> FMVSLPRMVYPQPKVL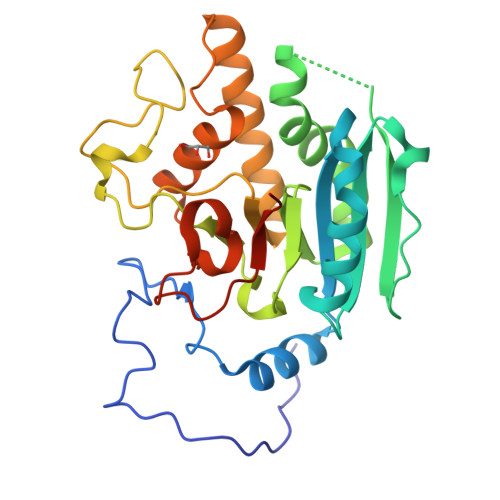TPCRKDVLVVTPWLAPIVWEGTFNIDILNEQFRLQNTTIGLTVFAIKKYVAFLKLFLETAEKHFMVGHRVHYYVFTDQPAAVPRVTLGTGRQLSVLEVGAYKRWQDVSMRRMEMISDFCERRFLSEVDYLVCVDVDMEFRDHVGVEILTPLFGTLHPSFYGSSREAFTYERRPQSQAYIPKDEGDFYYMGAFFGGSVQEVQRLTRACHQAMMVDQANGIEAVWHDESHLNKYLLRHKPTKVLSPEYLWDQQLLGWPAVLRKLRFTAVPKNHQAVRNPE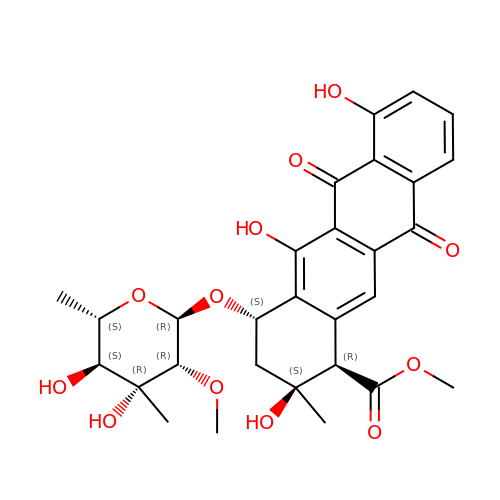3',4'-demethoxy-nogalose-nogalamycinone | C29 H32 O12 | XDICDWFRDRDUMQ-GUXZDVRLSA-N>STRSTVPNDDGVENHGGGTLFVTVQRCRNLKNKETIGVSDPYVKLQLRKQTRKSPYISSTLNPDFNFEAALEVYDIRSDVLHISILDKNDLVKDRLMGTLRIMLSQVAAAPGDIIRGDMNLDPEGQISLELKLLRH[2x]

Extended synaptotagmins (E-Syts) localize at membrane contact sites between the endoplasmic reticulum (ER) and the plasma membrane to mediate inter-membrane lipid transfer and control plasma membrane lipid homeostasis. All known E-Syts contain an N-terminal transmembrane (TM) hairpin, a central synaptotagmin-like mitochondrial lipid-binding protein (SMP) domain, and three or five C2 domains at their C termini. Here we report an uncharacterized E-Syt from the protist parasite Trypanosoma brucei, namely, TbE-Syt. TbE-Syt contains only two C2 domains (C2A and C2B), making it the shortest E-Syt known by now.

The structure was solved to 1.5 Å resolution using the selenium single-wavelength anomalous diffraction de novo phasing method. There are two molecules per asymmetric unit, both of which contain aa474-594 of TbE-Syt. The structure showed that TbE-Syt-C2B adopts a type II topology, consisting of eight β strands that form two sheets and a short α helix in the loop connecting β6 and β7. Additionally, there are two tightly bound Ca2+ ions, which are coordinated by a few charged residues in two extended loops on the opposite end from the helix. The interaction is mediated by a network of hydrogen bonds between the Ca2+ ions and the side-chain oxygens of residues E492, D498, D545, and N547, which are all highly conserved in trypanosomes. The main-chain carboxyl oxygens of residues V496 and K546 also form hydrogen bonds with either of the two Ca2+ ions. Similar to the Ca2+-binding site in the C2A domain of HsE-Syt2, TbE-Syt-C2B also has an extremely acidic “crater” on its surface. In the TbE-Syt-C2B structure there is also a basic patch on β2 and β3, which contains residues K502 and K511 at its center. Our structure-based mutagenesis studies revealed that TbE-Syt-C2B bound lipids in both Ca2+- and PI(4,5)P2-dependent manners via an acidic patch and an extended basic patch, respectively. Superimposing TbE-Syt-C2B onto each of the three C2 domains of HsE-Syt2 showed that it is very similar to HsE-Syt2-C2A and C2B, with average RMSDs of 1.05 Å and 0.75 Å, respectively, but substantially deviated from C2C, with an RMSD of 3.57 Å.> DTSHHDQDHPTFNKITPNLAEFAFSLYRQLAHQ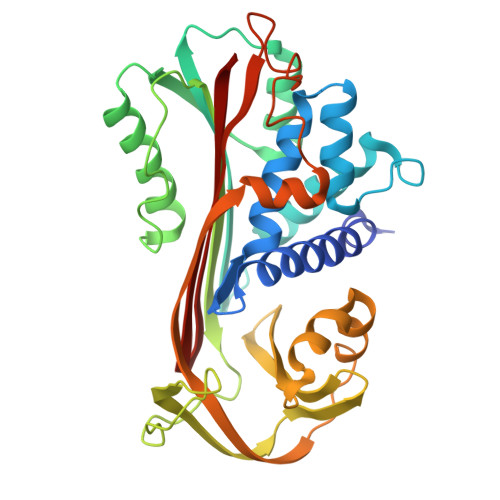SNSTNIFFSPVSIATAFAMLSLGTKADTHDEILEGLNFNLTEIPEAQIHEGFQELLRTLNQPDSQLQLTTGNGLFLSEGLKLVDKFLEDVKKLYHSEAFTVNFGDTEEAKKQINDYVEKGTQGKIVDLVKELDRDTVFALVNYIFFKGKWERPFEVKDTEEEDFHVDQVTTVKVPMMKRLGMFNIQHCKKLSSWVLLMKYLGNATAIFFLPDEGKLQHLENELTHDIITKFLENEDRRSASLHLPKLSITGTYDLKSVLGQLGITKVFSNGADLSGVTEEAPLKLSKAVHKAVLTIDEKGTEAAGAMFLEAIPM> MNDETLTVYRGATDNKGNPNKQVHGTVKGVFAWGPGTSTNKFGRDRNFKGESSSLTAELYVKRGADLKARDRIRRANGEEYSVVGHAAWDQGHPFDGFDFGYMVFQVEAVN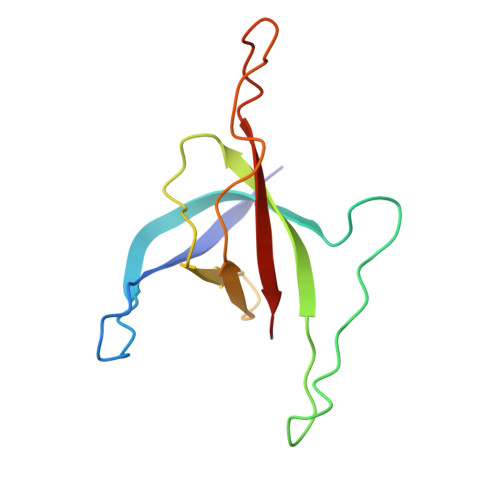A>[4x]KHPPLPFIKDQTLYERVFVHKSVVNGKTYLDQNDLINSHNERLEFLGDSVLNNLVTLIIYDKFPSASEGKLTKMRSQLIDNHTLTQ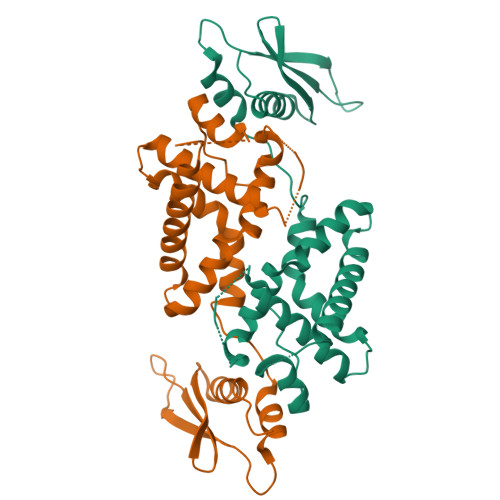FSFEYGFDKRLKTKTDEEILKTGDQKVYADIFEAYIGALSVERGLDLREIKDWLEKLYAPKLEAFKVNFLQESVNKEAKSELYSIVGTASSHPLYVVVEEGNGSHDFVVECRMGNDVLGRAKAPSQKEAGLRAAMDALKNRQLLE>MGSSHHHHHHSSGHSQSHGPSFISKGSKEYNGMKRDPLLDPTGEPEGHLWRADDNDYAPNSAHSARTNAALISLVRNEELEDLISTMKDLERTWNSKFNYPWIFFNDKPFTEEFKKRTQAETKAKCYYEQVPKEHWDPPEWINMELFRESAAILTEQKIQYSDKLSYHQMCRWNSGMFYKHPALKNYKYYWRVEPKVQFFCNVDYDVFRFMEDRNLTYGFTINLFDDPKTVPTLWPETKKFLA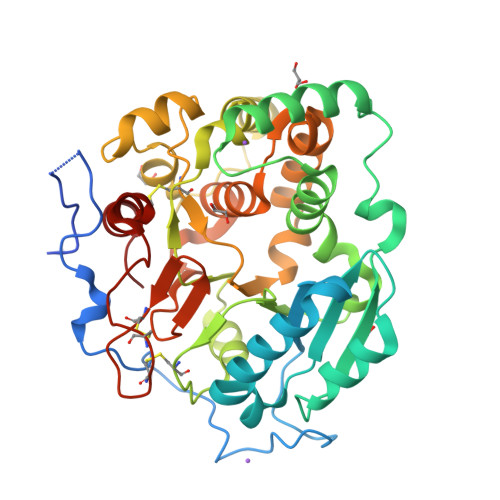ANPSYLSSNNMMGWLTDDSLRPDHTEAANGYSTCHFWSNFEIGDLDFFRGEQYDAYFNHLDRAGGFFYERWGDAPVHSIGLGLFADAAKVHWFRDIGYNHIPYYNCPNSPKCSKCTPGQFYAGAPFLAKEDCRPSYFKHVGMH[6x]>MTDTHTGPTPADAVPAYPFSLPHALDLDPHYAELRRDEPVSRVRLPYGEGTAWLVTRMSDARIVLGDSRFSTAAATDPATPRMFPTPPEPDGVLAQDPPDHTRLRRLVGKAFTARRVEEMRPRVRSLVDSLLDDMVAHGSPADLVEFLAVPFPVAVICELLGVPLEDRDLFRTFSDAMLSSTRLTAAEIQRVQQDFMVYMDGLVAQRRDAPTEDLLGALALATDNDDHLTKGEIVNMGVSLLIAGHETSVNQITNLVHLLLTERKRYESLVADPALVPAAVEEMLRYTPLVSAGSFVRVA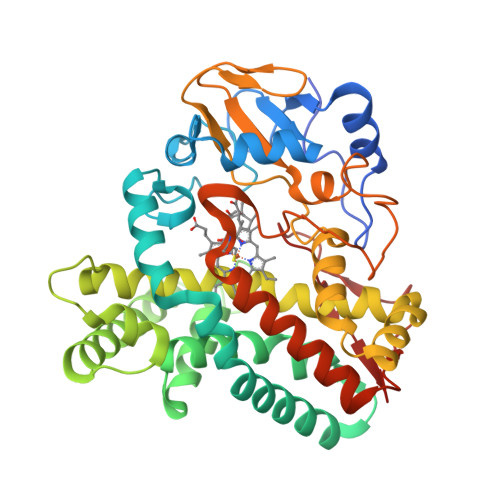TEDVELSTVTVRAGEPCVVHFASANRDEEVFDHADELDFHRERNPHIAFGHGAHHCIGAQLGRLELQEALSALVRRFPTLDLAEPVAGLKWKQGMLIRGLERQIVSW[9x]>[4x]MGSSHHHHHHSSGENLYFQGHMSNTSWRKSEVLAVPLQPTLQQEVILARMEQILASRALTDDERAQLLYERGVLYDSLGLRALARNDFSQALAIRPDMPEVFNYLGIYLTQAGNFDAAYEAFDSVLELDPTYNYAHLNRGIALYYGGRDKLAQDDLLAFYQDDPNDPFRSLWLYLAEQKLDEKQAKEVLKQHFEKSDKEQWGWNIVEFYLGNIS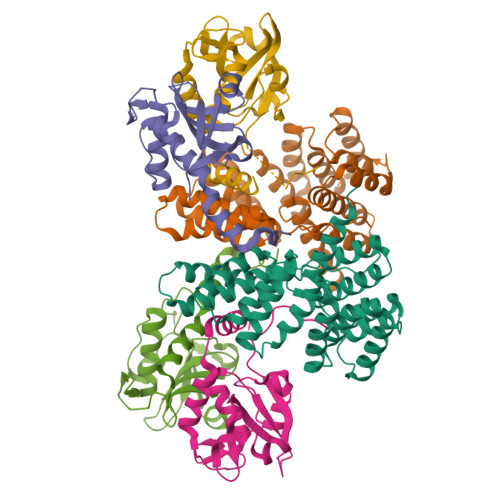EQTLMERLKADATDNTSLAEHLSETNFYLGKYYLSLGDLDSATALFKLAVANNVHNFVEHRYALLELSLLGQDQDDLAESDQQ;>MSANNTAKNMHPETRAVGSETSSLQASQDEFENLVRNVDVKSRIMDQYADWKGVRYRLGGSTKKGIDCSGFVQRTFREQFGLELPRSTYEQQEMGKSVSRSNLRTGDLVLFRAGSTGRHVGIYIGNNQFVHASTSSGVIISSMNEPYWKKRYNEARRVLSRSHHHHHH[8x]> MNNWQHFFNNPVDLSEHLKKPYFRFDNRDKEITAISFDEKANLIWSGDSYGCISSYDPTFQLYTRYRGHIGGNSVKDILSHRDGILSISEDSLHFANRRGVTKLNLTSIDIAAFSELNTMCYSPHSLKNNIYCGGDNTNWGIASIDLNRGCLDSLLNYSSKVKLMCSNNKVLSIGRQTGTVDLLDPTSNRTIKSFNAHSASISAMDLRDNTLVTVGKSKRFYNLYADPFVNVYDLRTMRQLPPVSFSKGTTMGSGGADFVQLHPLLPTVMIVASSSGSFDFIDLSNPTLRTQYVHPCQSIKKLCLSPNGDVLGILEADNHLDTWRRSSNNMGMFTNTPEMLAYPDYFNDITSDGPISVDDETYPLSSVGMPYYLDKLLSAWPPVVFKSEGTIPQLTGKSPLPSSGKLKSNLAVISSQNEKLSTQEFPLLRYDRTKYGMRNAIPDYVCLRDIRKQITSGLETSDIQTYTSINKYEVPPAYSRLPLTSGRFGTDNFDFTPFNNTEYSGLDPDVDNHYTNAIIQLYRFIPEMFNFVVGCLKDENFETTLLTDLGYLFDMMERSHGKICSSSNFQASLKSLTDKRQLENGEPQEHLEEYLESLCIRESIEDFNSSESIKRNMPQKFNRFLLSQLIKEEAQTVNHNITLNQCFGLETEIRTECSCDHYDTTVKLLPSLSISGINKTVIKQLNKKSNGQNILPYIEYAMKNVTQKNSICPTCGKTETITQECTVKNLPSVLSLELSLLDTEFSNIRSSKNWLTSEFYGSIIKNKAVLRSTASELKGTSHIFKYELNGYVAKITDNNNETRLVTYVKKYNPKENCFKWLMFNDYLVVEITEEEALKMTYPWKTPEIIIYCDAEELRKPFFSVDTYSIN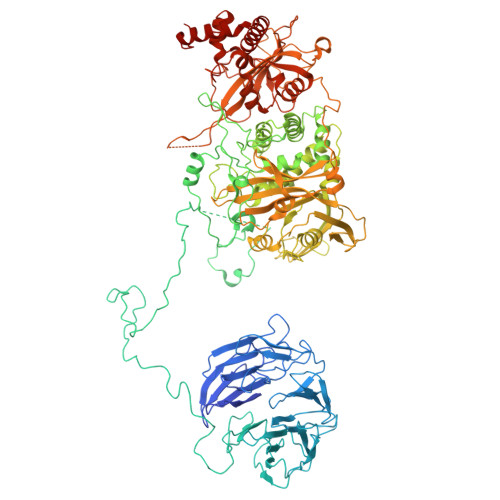YDILFRDYFANGIRDTARREYKLLTHDEAPKSGTLVAIDAEFVSLQSELCEIDHQGIRSIIRPKRTALARISIIRGEEGELYGVPFVDDYVVNTNHIEDYLTRYSGILPGDLDPEKSTKRLVRRNVVYRKVWLLMQLGCVFVGHGLNNDFKHININVPRNQIRDTAIYFLQGKRYLSLRYLAYVLLGMNIQEGNHDSIEDAHTALILYKKYLHLKEKAIFEKVLNSVYEEGRAHNFKVPETSKG> MFQDVLVITVAAGRGGDGAVSFRREKFVPKGGPDGGDGGRGGSVYLRARGSVDSLSRLSKRTYKAEDGEHGRGSQQHGRGGEDLVIEVPRGTRVFDADTGELLADLTEEGQTVLV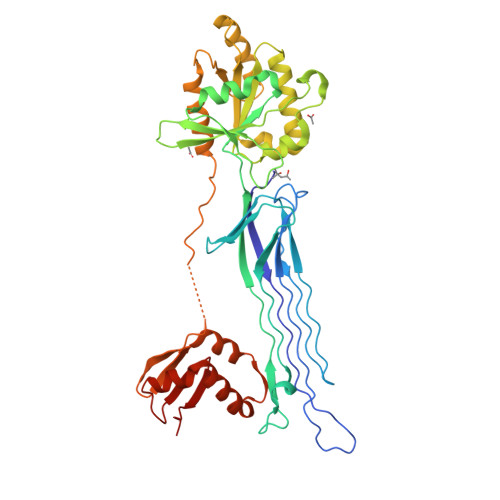ARGGAGGRGNMHFVSPTRQAPRFAEAGEEGEKRRLRLELMLIADVGLVGYPNAGKSSLLAAMTRAHPKIAPYPFTTLSPNLGVVEVSEEERFTLADIPGIIEGASEGKGLGLEFLRHIARTRVLLYVLDAADEPLKTLETLRKEVGAYDPALLRRPSLVALNKVDLLEEEAVKALADALAREGLAVLPVSALTGAGLPALKEALHALVRSTPPPEMPKPVPRKEVQAGVEVVPVAEGVYEVRAPEVERYLARIKGDLMEAAGYLQEVFRRQGVEAALRAKGVRAGDLVRIGGLEFEYIPEV>MWKRSEQMKIKSGKCNMAAAMETEQLGVEIFETADCEENIESQDRPKLEPFYVERYSWSQLKKLLADTRKYHGYMMAKAPHDFMFVKRNDPDGPHSDRIYYLAMSGENRENTLFYSEIPKTINRAAVLMLSWKPLLDLFQATLDYGMYSREEELLRERKRIGTVGIASYDYHQGSGTFLFQAGSGIYHVKDGGPQGFTQQPLRPNLVETSCPNIRMDPKLCPADPDWIAFIHSNDIWISNIVTREERRLTYVHNELANMEEDARSAGVATFVLQEEFDRYSGYWWCPKAETTPSGGKILRILYEENDESEVEIIHVTSPMLETRRADSFRYPKTGTANPKVTFKMSEIMIDAEGRIIDVIDKELIQPFEILFEGVEYIARAGWTPEGKYAWSILLDRSQTRLQIVLISPELFIPVEDDVMERQRLIESVPDSVTPLIIYEETTDIWINIHDIFHVFPQSHEEEIEFIFASECKTGFRHLYKITSILKESKYKRSSGGLPAPSDFKCPIKEEIAITSGEWEVLGRHGSNIQVDEVRRLVYFEGTKDSPLEHHLYVVSYVNPGEVTRLTDRGYSHSCCISQHCDFFISKYSNQKNPHCVSLYKLSSPEDDPTCKTKEFWATILDSAGPLPDYTPPEIFSFESTTGFTLYGMLYKPHDLQPGKKYPTVLFIYGGPQVQLVNNRFKG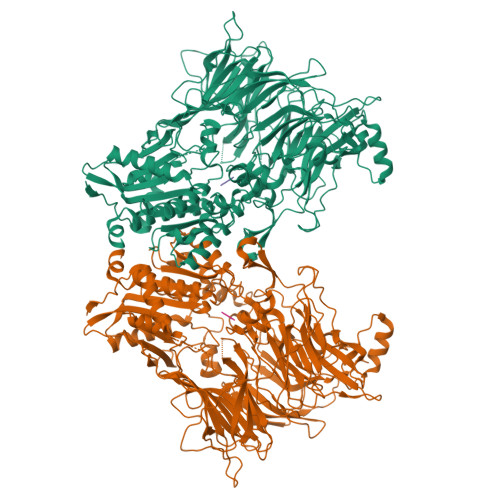VKYFRLNTLASLGYVVVVIDNRGSCHRGLKFEGAFKYKMGQIEIDDQVEGLQYLASRYDFIDLDRVGIHGWSYGGYLSLMALMQRSDIFRVAIAGAPVTLWIFYDTGYTERYMGHPDQNEQGYYLGSVAMQAEKFPSEPNRLLLLHGFLDENVHFAHTSILLSFLVRAGKPYDLQIYPQERHSIRVPESGEHYELHLLHYLQENLGSRIAALKVI[3x];>MP[3x]> GAASNKSTSSA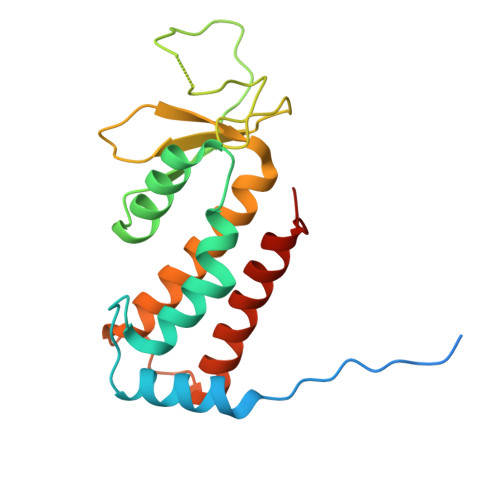MSGSHQDLSVIQPIVKDCKEADLSLYNEFRLWKDEPTMDRTCPFLDKIYQEDIFPCLTFSKSELASAVLEAVENNTLSIEPVGLQPIRFVKASAVECGGPKKCALTGQSKSCKHRIKLGDSSNYYYISPFCRYRITSVCNFFTYIRYIQQGLVKQQDVDQMFWEVMQLRKEMSLAKLGYFKEEL ACRIDINE 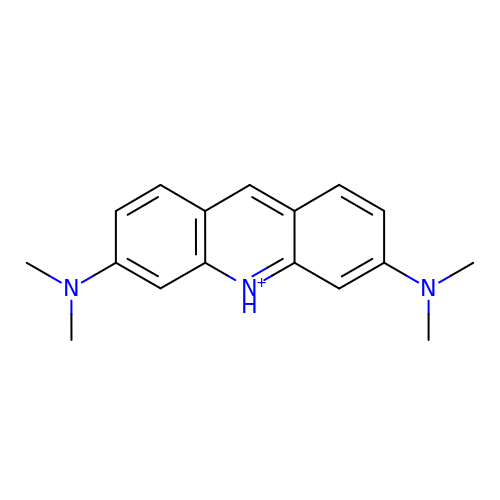ORANGE | C17 H20 N3 | DPKHZNPWBDQZCN-UHFFFAOYSA-O>[4x]TTIHDVQTTGLTQDAV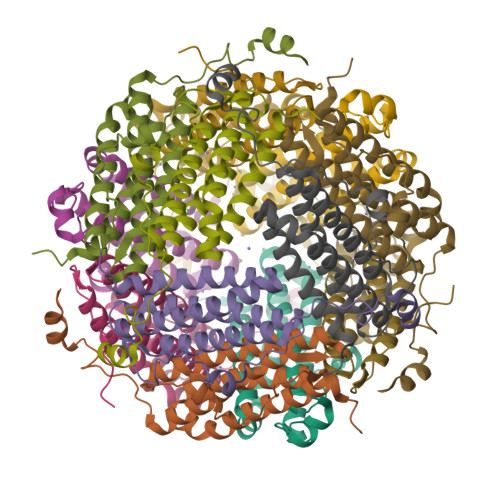TGFDASSRLNAGLQEVLVDLTALHLQGKQAHWNIVGENWRDLHLQLDTLVEAARGFSDDVAERMRAVGGVPDARPQTVAASRIGDVGPDEIDTRACVEAIVALVRHTVDTIRRVHDPIDAEDPASADLLHAITLELEKQAWMIGSENRSPRRR> MPSSLLGAAMPASTSAAALQEALENAGRLIDRQLQEDRMYPDLSELLMVSAPNNPTVSGMSDMDYPLQGPGLLSVPNLPEISSIRRVPLPPELVEQFGHMQCNCMMGVFPPISRAWLTIDSDIFMWNYEDGGDLAYFDGLSETILAVGLVKPKAGIFQPHVRHLLVLATPVDIVILGLSYANLQTGSGVLNDSLSGGMQLLPDPLYSLPTDNTYLLTITSTDNGRIFLAGKDGCLYEVAYQAEAGWFSQRCRKINHSKSSLSFLVPSLLQFTFSEDDPILQIAIDNSRNILYTRSEKGVIQVYDLGQDGQGMSRVASVSQNAIVSAAGNIARTIDRSVFKPIVQIAVIENSESLDCQLLAVTHAGVRLYFSTCPFRQPLARPNTLTLVHVRLPPGFSASSTVEKPSKVHRALYSKGILLMAASENEDNDILWCVNHDTFPFQKPMMETQMTAGVDGHSWALSAIDELKVDKIITPLNKDHIPITDSPVVVQQHMLPPKKFVLLSAQGSLMFHKLRPVDQLRHLLVSNVGGDGEEIERFFKLHQEDQACATCLILACSTAACDREVSAWATRAFFRYGGEAQMRFPTTLPPPSNVGPILGSPVYSSSPVPSGSPYPNPSFLGTPSHGIQPPAMSTPVCALGNPATQATNMSCVTGPEIVYSGKHNGICIYFSRIMGNIWDASLVVERIFKSGNREITAIESSVPCQLLESVLQELKGLQEFLDRNSQFAGGPLGNPNTTAKVQQRLIGFMRPENGNPQQMQQELQRKFHEAQLSEKISLQAIQQLVRKSYQALALWKLLCEHQFTIIVAELQKELQEQLKITTFKDLVIRDKELTGALIASLINCYIRDNAAVDGISLHLQDICPLLYSTDDAICSKANELLQRSRQVQNKTEKERMLRESLKEYQKISNQVDLSNVCAQYRQVRFYEGVVELSLTAAEKKDPQGLGLHFYKHGEPEEDIVGLQAFQERLNSYKCITDTLQELVNQSKAAPQSPSVPKKPGPPVLSSDPNMLSNEEAGHHFEQMLKLSQRSKDELFSIALYNWLIQVDLADKLLQVASPFLEPHLVRMAKVDQNRVRYMDLLWRYYEKNRSFSNAARVLSRLADM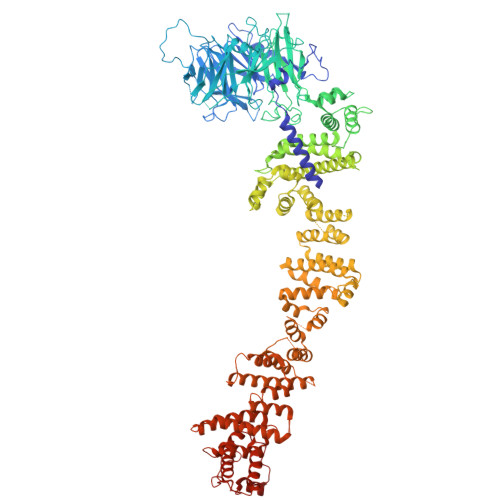HSTEISLQQRLEYIARAILSAKSSTAISSIAADGEFLHELEEKMEVARIQLQIQETLQRQYSHHSSVQDAVSQLDSELMDITKLYGEFADPFKLAECKLAIIHCAGYSDPILVQTLWQDIIEKELSDSVTLSSSDRMHALSLKIVLLGKIYAGTPRFFPLDFIVQFLEQQVCTLNWDVGFVIQTMNEIGVPLPRLLEVYDQLFKSRDPFWNRMKKPLHLLDCIHVLLIRYVENPSQVLNCERRRFTNLCLDAVCGYLVELQSMSSSVAVQAITGNFKSLQAKLERLH> XFDPPLHST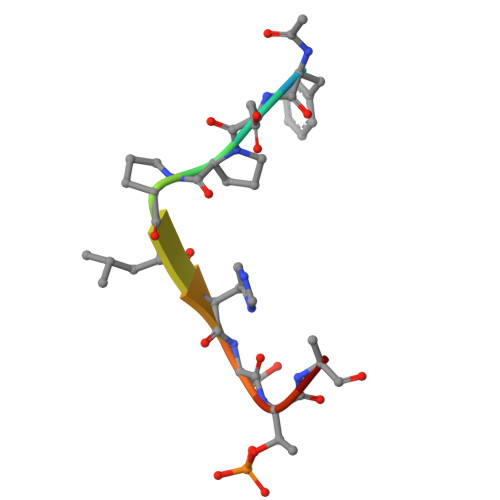AX> MKELIYIEEPKILFAHGQKCTDARDGLALFGPLNNLYGIKSGVIGTKQGLKIFRDYLDHIQKPIYNSNSITRPMFPGFEAVFDCKWESTGITFKEVTNEDIGKFLYNSSTHKRTYDLVSLFIDKIISANKNEDENVDVWFVIVPDEIYKYCRPNSVLPKEMVQTKALMSKSKAKSFRYEPSLFPDINIELKEQEKEAETYNYDAQFHDQFKARLLKHTIPTQIFRESTLAWRDFKNAFGLPIRDFSKIEGHLAWTISTAAFYKAGGKPWKLSDVRNGVCYLGLVYKKVEKSKNPRNACCAAQMFLDNGDGTVFKGEVGPWYNPKNGQYHLEPKEAKALLSQSLQSYKEQIGEYPKEVFIHAKTRFNHQEWDAFLEVTPKETNLVGVTISKTKPLKLYKTEGDYTILRGNAYVVNERSAFLWTVGYVPKIQTALSMEVPNP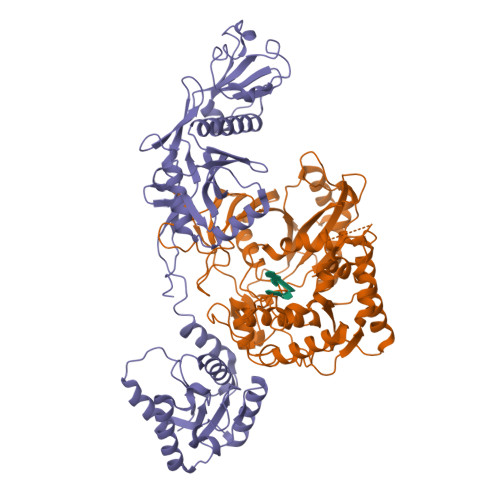LFIEINKGEADIKQVLKDILSLTKLNYNACIFADGEPVTLRFADKIGEILTASTDIKTPPLAFKYYI;> MRNKIFISHATPDDNDFTRWLALKLIGLGYEVWCDILFLDKGVDFWSNIEKVIREDTCKFLLVSSSYSNQREGVLKELAVAAKVKKQLKDDKFIIPLAIDEQLSYDDINIDIVRLNAIDFKMSWARGLKDILEAFEKQKVPKEVADASKSNLLYQQIFLHDKSVIEKEEIYDSNWLSILSFPEELRFHEYNWMLPKRFDVRELTFPAVRYKNYLCTFAWAYDFTYHLPKTETYHKSKTIRIPTEEILSGSYDSNFIRNAECKRLIVQLLNKAFELRMKDKEVQEYEMSNKTAYWLEKGKLEKDKFEKTMLVGKQKDKNWHFAISGASKLYPFPVLMISSHIFFTADGKKLIDSSSVQHSSRRRQGKNWWNNTWRTKLLAFIKYLSDDDTSFYLEMGSEEKVFVSNEPVKFKGNVSYNIPEKNTLEEEAELSGFNQGEDIEELEELIENLEAE> MQVNRLPFFTNHFFDTYLLISEDTP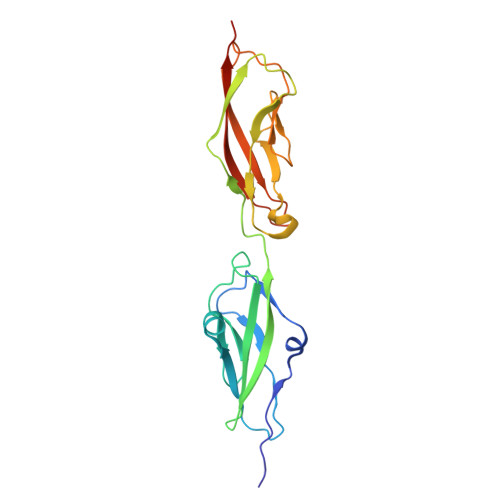VGSSVTQLLARDMDNDPLVFGVSGEEASRFFAVEPDTGVVWLRQPLDRETKSEFTVEFSVSDHQGVITRKVNIQVGDVNDNAPTFHNQPYSVRIPENTPVGTPIFIVNATDPDLGAGGSVLYSFQPPSPFFAIDSARGIVTVIQELDYEVTQAYQLTVNATDQDKTRPLSTLANLAIIITDLEHHHHHH> DNQFYSVEVGDSTFTVLKRYQNLKPIGSGAQGIVCAAYDAVLDRNVAIKKLSRPFQNQTHAKRAYRELVLMKCVNHKNIISLLNVFTPQKTLEEFQDVYLVMELMDANLCQVIQMELDHERMSYLLYQMLCGIKHLHSAGIIHRDLKPSNIVVKSDCTLKILDFGLARTAGTSFMMTPYVVTRYYRAPEVILGMGYKENVDIWSVGCIMGEMVRHKILFPGRDYIDQWNKVIEQLGTPCPEFMKKLQPTVRNYVENRPKYAGLTFPKLFPDSLFPADSEHNKLKASQARDLLSKMLVIDPAKRISVDDAL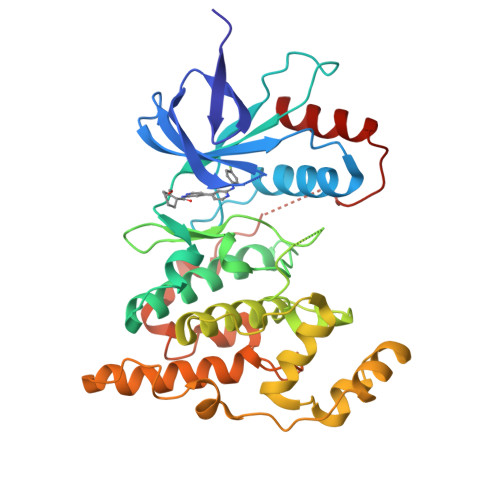QHPYINVWYDPAEVEAPPPQIYDKQLDEREHTIEEWKELIYKEVMN>MSLLSDLCNLNLSESTEKIIAEYIWIGGSGMDLRSKARTLNAPVSDPSKLPQWNYDGSSTGQAPGEDSEVILYPQAIYKDPFRRGNNILVMCDAYTPGGEPIPTNKRFDAAKIFSHPDVVAEEPWYGIEQEYTLLQKEVKWPIGWPVGGYPGPQGPYYCGIGADKAFGRDIVDAHYKACLYAGINISGINGEVMPGQWEFQVGPSVGISSGDQLWMARYILERITEIAGVVVSFDPKPIEGDWNGAGAHTNYSTKSMRSDGGFEVIKKAIEKLGLKHREHIAAYGEGNERRLTGKHETADINTFLWGVANRGASIRVGRDTEKAGKGYFEDRRPASNMDPYIVTSMIANTTILWKP[10x]

One such an example is glutamine synthetases (GSs) (EC 6.3.1.2), one of the most ancient functioning enzymes in existence and a central enzyme in nitrogen metabolism of all living organisms, catalyzing the formation of glutamine by condensation of glutamate with ammonia using ATP as an energy source. Decades of studies have established a striking notion that all three classes of GS enzymes, despite of dramatic differences in amino acid sequences and protein sizes, share quaternary geometry in dihedral symmetry assembled with two oligomeric rings. Considering that the active sites of GS are located at the clefts formed between two neighboring protomers within the same ring and distal to the ring-ring interface, each isolated GS subcomplex ring holds multiple integral catalytic sites. Cryo-EM structure determination of GS in both the catalytically active and inactive assembly states allows us to reveal an unanticipated self-assembly-induced disorder-order transition paradigm, in which the remote interactions between two subcomplex entities significantly rigidify the otherwise structurally fluctuating active sites, thereby regulating activity.

In contrast, under the same condition the majority fraction (~82%) of CsGSIb adopts a pentameric configuration, along with a minor fraction (~18%) being decameric. To elucidate the detailed mechanism of how the interactions between two GSII pentameric rings remotely trigger enzymatic activity, we next employed single-particle cryo-EM imaging technique and first determined the structures of GmGSβ2 decamer, as well as that of the CsGSIb that adopts decameric configuration (thereafter named as CsGSIbDec). 3D classifications of 104,717 and 43,876 particles for GmGSβ2 and CsGSIbDec, respectively, revealed that both molecules were arranged in D5 symmetry with two pentameric rings stacked in a head-to-head manner, a strikingly conserved structural feature for type II GS species. Refinement of the GmGSβ2 and CsGSIbDec structures yielded maps with an average resolution of 2.9 Å and 3.3 Å, respectively (Figure 3—figure supplements 1–3), with literally identical dimensions of 115 Å x 115 Å x 95 Å. The active sites of GmGSβ2, CsGSIbDec are structurally highly similar to each other, as well as to that of the maize GSII, suggesting the catalysis mechanisms of these plant GSIIs are essentially identical. The overall buried inter-ring surfaces for both GmGSβ2 and CsGSIbDec amount to ~2000 Å2, that is approximately only 400 Å2 per individual monomer–monomer interaction. This highlights the weakness of the inter-ring contacts, characteristic of type II GS. Indeed, in both structures the inter-ring contacts are established by only a limited number of hydrophobic and polar interactions provided by the residues 136–141 and 146–152 segments of each of the intervening subunits, which behave as two gear teeth (thereafter named as tooth-1 and tooth-2, respectively) interlocking the two pentameric rings.>MRGSHHHHHHGSMSVSEIFVELQGFLAAEQDIREEIRKVVQSLEQTAREILTLLQGVHQGAGFQDIPKRCLKAREHFGTVKTHLTSLKTKFPAEQYYRFHEHWRFVLQRLVFLAAFVVYLETETLVTREAVTEILGIEPDREK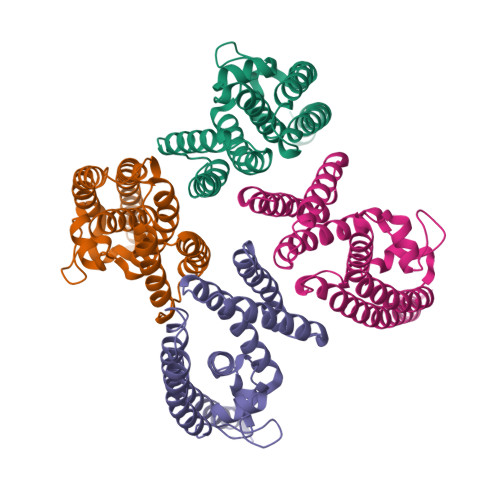GFHLDVEDYLSGVLILASELSRLSVNSVTAGDYSRPLHISTFINELDSGFRLLNLKNDSLRKRYDGLKYDVKKVEEVVYDLSIRGFNKETAAACVEK[4x]> MVSAADVYVPDEWEVAREKITMSRELGQGSFGMVYEGVAKGVVKDEPETRVAIKTVNEAASMRERIEFLNEASVMKEFNCHHVVRLLGVVSQGQPTLVIMELMTRGDLKSYLRS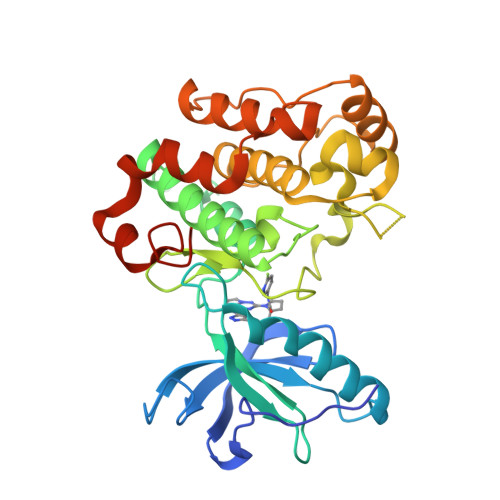LRPEMENNPVLAPPSLSKMIQMAGEIADGMAYLNANKFVHRDLAARNCMVAEDFTVKIGDFGMTRDIYETDYYRKGGKGLLPVRWMSPESLKDGVFTTYSDVWSFGVVLWEIATLAEQPYQGLSNEQVLRFVMEGGLLDKPDNCPDMLFELMRMCWQYNPKMRPSFLEIISSIKEEMEPGFREVSFYYSEENKMENNPVLA> CGGPFELWEPNTTFSSTNFPNSYPNLAFCVWILNAQKGKNIQLHFQEFDLENINDVVEIRDGEEADSLLLAVYTGPGPVKDVFSTTNRMTVLLITNDVLARGGFKANFTTGYHLGIPEPCKADHFQCKNGECVPLVNLCDGHLHCEDGSDEADCVRFFNGTTNNNGLVRFRIQSIWHTACAENWTTQISNDVCQLLGLGSGNSSKPIFPTDGGPFVKLNTAPDGHLILTPSQQCLQDSLIRLQCNHKSCGKKLAAQDITPK;> IVGGSNAKEGAWPWVVGLYYGGRLLCGASLVSSDWLVSAAACVYGRNLEPSKWTAILGLHMKSNLTSPQTVPRLIDEIVINPHYNRRRKDNAIAMMHLEFKVNYTDYIQPICLPEENQVFPPGRNCSIAGWGTVVYQGTTANILQEADVPLLSNERCQQQMPEYNITENMICAGYEEGGIDSCQGDAGGPLMCQENNRWFLAGVTSFGYKCALPNRPGVYARVSRFTEWIQSFLH

Human enteropeptidase (hEP), also known as enterokinase, is an essential enzyme in food digestion and is localized at the brush border of the duodenal and jejunal mucosa. Activated hEP can stimulate the conversion of trypsinogen to trypsin via cleavage of a specific trypsinogen activation peptide, namely Asp-Asp-Asp-Asp-Lys (DDDDK), which is highly conserved in vertebrates. However, the mechanism of hEP activation remains to be established. hEP contains a multi-domain heavy chain and a catalytic light chain, linked by a disulfide bond. The functions of these domains and motifs may be involved in protein anchoring, macromolecular substrate recognition and inhibitor specificity. The light chain is homologous to trypsin-like serine proteinases with a typical Asp-His-Ser (D-H-S) catalytic triad responsible for peptidase activity.

We mutated all three residues to Ala (namely hEPmut) and observed the abolished proteolytic activity even in the active state. Notably, native gel analysis showed a reduced shift of the mutated hEP core (hEPmut-core) compared to the wild-type hEP core (hEPwt-core) upon activation, likely caused by a change in charge. To investigate the influence of charge on the catalytic pocket arrangement, we determined the active hEPmut-core structure at a resolution of 3.7 Å. The overall architectures and the catalytic triads of active hEPmut, and hEPwt cores were quite similar, with an r.m.s. deviation of 0.799 Å, indicating that mutation of the catalytic triad abolished the catalytic activity without changing the catalytic pocket. In conclusion, our study revealed an activation mechanism of hEP involving a flipping of the IVGG loop to stabilize the surface loops around the catalytic sites; our results also suggested the surface charge provided by the catalytic triad to have no effect on hEP activation, but it may affect the catalytic substrate reaction by reducing substrate binding affinity. However, the active hEPmut alone can generate a normal hEP map, showing an overall shape equivalent to that of the active hEPwt with a well-organized catalytic pocket.> 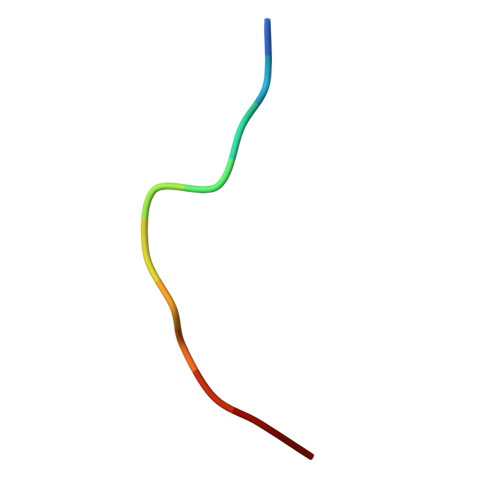PYVPVHFDASV>[4x]MPTLGLLFASIGIAVLAMGVPHCRGYTIKEDESFLQQPHYASQEQLEDLFAGLEKAYPNQAKVHFLGRSLEGRNLLALQISRNTRSRNLLTPPVKYIANMHGDETVGRQLLVYMAQYLLGNHERISDLGQLVNSTDIYLVPTMNPDGYALSQEGNCESLPNYVGRGNAANIDLNRDFPDRLEQSHVHQLRAQS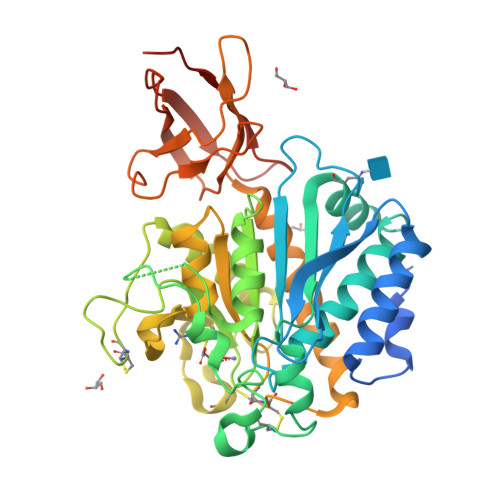RQPETAALVNWIVSKPFVLSANFHGGAVVASYPYDNSLAHNECCEESLTPDDRVFKQLAHTYSDNHPIMRKGNNCNDSFSGGITNGAHWYELSGGMQDFNYAFSNCFELTIELSCCKYPAASTLPQEWQRNKASLLQLLRQAHIGIKGLVTDASGFPIADANVYVAGLEEKPMRTSKRGEYWRLLTPGLYSVHASAFGYQTSAPQQVRVTNDNQEALRLDFKLAPVETNFDGISSFYSPYYF>[4x]MAHSKHGLKEEMTM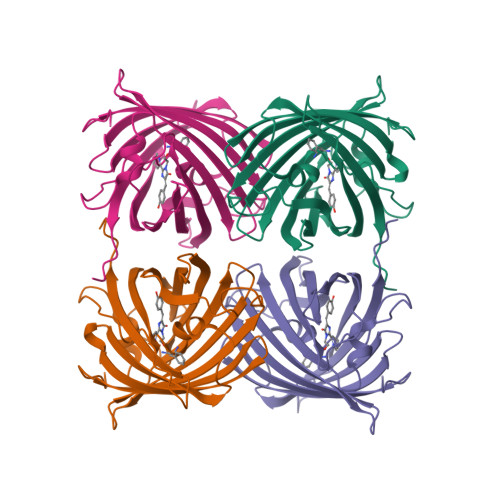KYHMEGCVNGHKFVITGEGIGYPFKGKQTINLCVIEGGPLPFSEDILSAGFKYGDRIFTEYPQDIVDYFKNSCPAGYTWGRSFLFEDGAVCICNVDITVSVKENCIYHKSIFNGMNFPADGPVMKKMTTNWEASCEKIMPVPKQGILKGDVSMYLLLKDGGRYRCQFDTVYKAKSVPSKMPEWHFIQHKLLREDRSDAKNQKWQLTEHAIAFPSALA>[2x]MATSVQTGKAKQLTLLGFFAITASMVMAVYEYPTFATSGFSLVFFLLLGGILWFIPVGLCAAEMATVDGWEEGGVFAWVSNTLGPRWGFAAISFGYLQIAIGFIPMLYFVLGALSYILKWPALNEDPITKTIAALIILWALALTQFGGTKYTARIAKVGFFAGILLPAFILIALAAIYLHSGAPVAIEMDSKTFFPDFSKVGTLVVFVAFILSYMGVEASATHVNEMSNPGRDYPLAMLLLMVAAICLSSVGGLSIAMVIPGNEINLSAGVMQTFTVLMSHVAPEIEWTVRVISALLLLGVLAEIASWIVGPSRGMYVTAQKNLLPAAFAKMNKNGVPVTLVISQLVITSIALIILTNTGGGNNMSFLIALALTVVIYLCAYFMLFIGYIVLVLKHPDLKRTFNIPGGKGV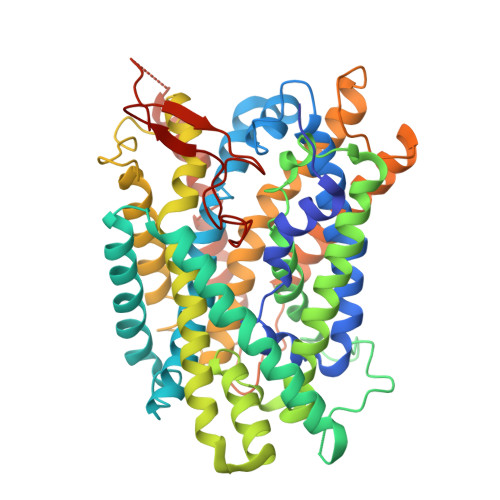KLVVAIVGLLTSIMAFIVSFLPPDNIQGDSTDMYVELLVVSFLVVLALPFILYAVHDRKGKANTGVTLEPINSQNAPKGHFFLHPRARSPHYIVMNDKKH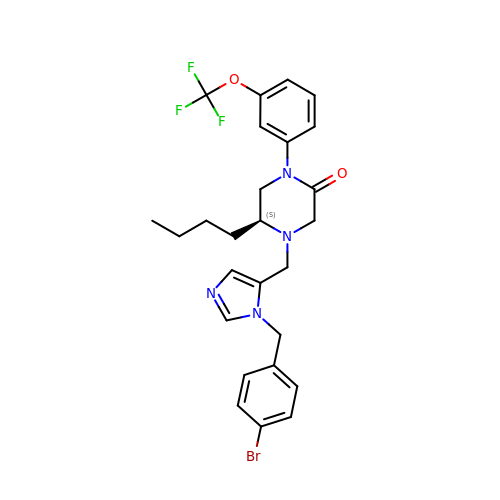(5S)-4-({1-[(4-bromophenyl)methyl]-1H-imidazol-5-yl}methyl)-5-butyl-1-[3-(trifluoromethoxy)phenyl]piperazin-2-one | C26 H28 Br F3 N4 O2 | GQAHQWQDBPUSHR-QFIPXVFZSA-N> GPAMAGNLYGRDGAAIGSLQKLRFFPLAVAGGQGARLVEEDGRELIDLSGAWGAASLGYGHPAIIEAVSRAAANPAGASILSASNAPAVALAERLTA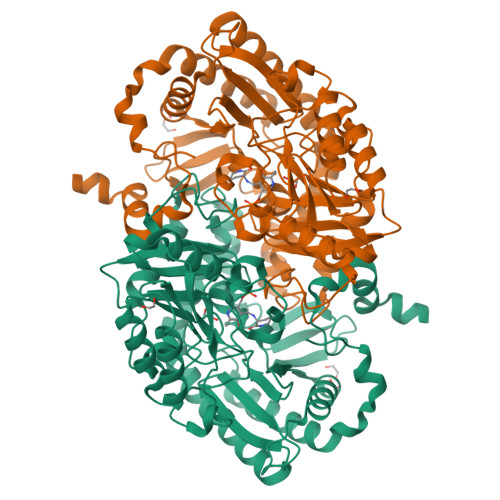SFPGRGTHKVWFGHSGSDANEAAYRAITRATGRTGVIAFIGAYHGCTVGSMAFSGHSVQADAAKADGLILLPYPDPYRPYQDDPTGDAVLALLKERLAAVPAGSIAAAFIEPIQSDGGLIVPPDGFLRKFADICRAHGISVVCDEVAVGLARSGRLHCFEHEGFVPDILVLGKGLGGGLPLSAVIAPAEILDCASAFAMQTLHGNPVCAAAGLAVLETIEAENLTTAAERKGKLLREGLARLAERHELIGDIRGRGLACGVELVRNRQSREPARAETAKLIYRAYELGLVLYYVGMNGNVLEMTPPLTMTEDEVRHAVNLLDQAFTELSTVSDTLVSQFAGW> PAERLHSLFARADVLAHLLHSRLALPLLYPLNSGGALTNPLNSAASPDSPAALNSIATSRWKREEVMSALATVTPLVLAATSVSRFLKTAHALSY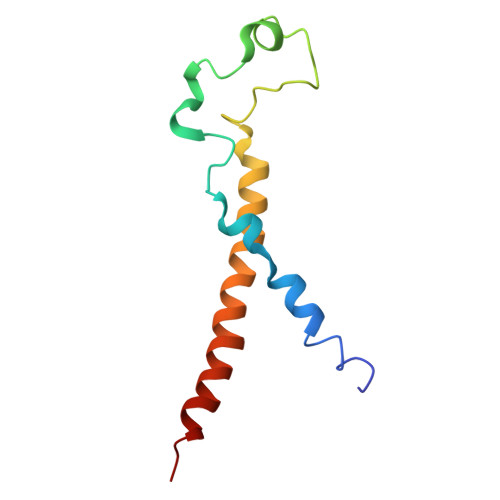FA> GEPLYTEQDLAVNGREGFPNYSHPALTVTPDGDLLASYDGRPTGIAAPGPNSILQRRSTDGGRTWGEQQVVSAGQTTAPIKGFSHPSYLVDRETGTIFNFHVYSQRQGWEGSRPGTDPADPNVLHANVAT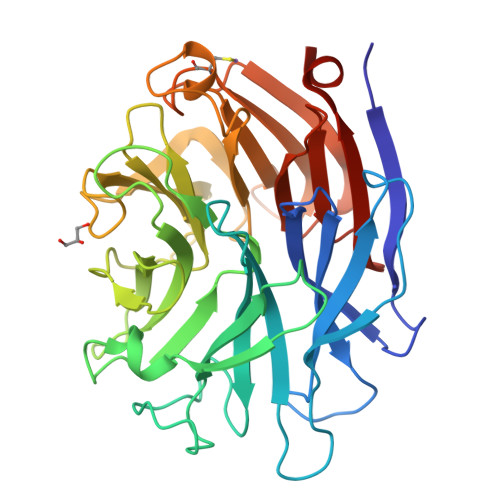STDGGLTWSHRTITADITPDPGWRSRFAASGEGIQLRYGPHAGRLIQQYAIINAAGAIQAVSVYSDDHGRTWRAGEAVGVGMSHNKTVELSDGRVLLNSADSARSGYRKVAVSTDGGHSYGPVTIDRDLPDPTNDASIIRAFPDAPAGSARAKVLLFSNAASQTSRSQGTIRMSCDDGQTWPVSKVFQPGSMSYSTLTALPDGTYGLLYEPGTGIRYANFNLAWLGGICAPGS> GIPATGDGACLFNAVSIGLSVEILSGRLDSQLDTPGYQALLDEFAKHHPQFNPKSWKTLKEWLAYYNDTRDIELILAPVLFNLNQKYQDHLDEEILNELTNLVWKNKANIENGQAWFQLQNTGDLGEALFPKLENLDLKKDRAPLLDKLREILKDYKLELTRENVKQFLTEKAKELLSALKKKISSDPHAFQRGYSCDELKGMTDALAISLVENREEDITDNRIKIRLENQEEH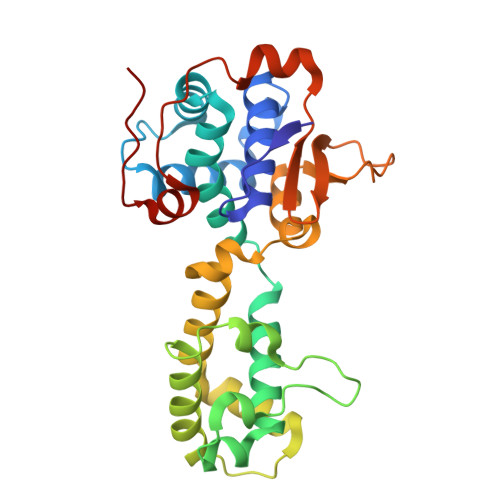WNVLCNEEDSERFLDSTPSRLKMTSLEAYRGDKQVSAPT> MKALLPGLYLLPVPIPYPLKTVNLYLLQGAGEVALVDTALGTRAARGALELHLAELGLCFQDVKTILLTHHHPDHYGLSGFFEGLGARVFLHEEEFARGHRFWREPEAFAEASWRLFLDHGTPEGALQGIRETVEKTRERVHPPQNPLPLRDGEALEVAGKRLRVLWTPGHADGHAAFYLEEEGVLLAGDALLEKVSPNVGLWAYTRENPLKDFLRSLDRLADLGARV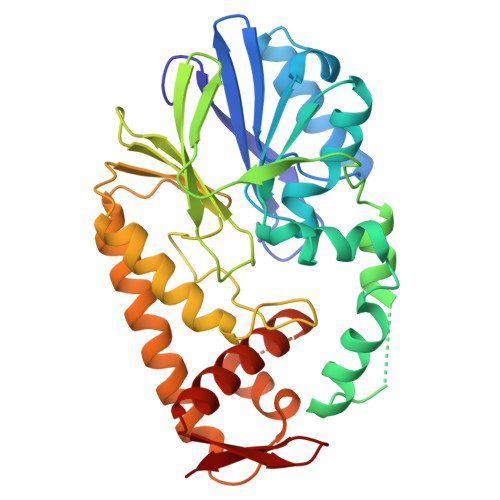AYAGHFGPIADVRQRAEELKAHHQARLEALLALLDGPKTAWELSLHLFPQELDPAGRRFAFAETLAHLEYLREEGAVGRGGPPYRYFRR> RRRQRSAVQQLQPTQAGISMAPSAQGAMVRIRNPAVSSSRGG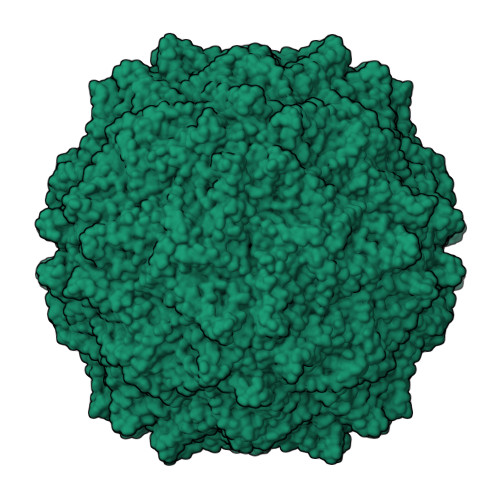ITVLTHSELSAEIGVTDSIVVSSELVMPYTVGTWLRGVAANWSKYSWLSVRYTYIPSCPSSTAGSIHMGFQYDMADTVPVSVNQLSNLRGYVSGQVWSGSAGLCFINGTRCSDTSTAISTTLDVSKLGKKWYPYKTSADYATAVGVDVNIATPLVPARLVIALLDGSSSTAVAAGRIYCTYTIQMIEPTASALNN> KPVIKMYQIGDKPDNLDELLANANKIIEEKVGAKLDIQYLGWGDYGKKMSVITSSGENYDIAFADNYIVNAQKGAYADLTELYKKEGKDLYKALDPAYIKGNTVNGKIYAVPVAANVASSQNFAF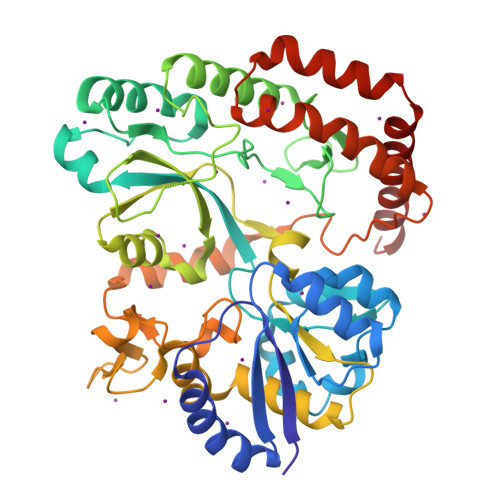NGTLLAKYGIDISGVTSYETLEPVLKQIKEKAPDVVPFAIGKVFIPSDNFDYPVANGLPFVIDLEGDTTKVVNRYEVPRFKEHLKTLHKFYEAGYIPKDVATSDTSFDLQQDTWFVREETVGPADYGNSLLSRVANKDIQIKPITNFIKKNQTTQVANFVISNNSKNKEKSMEILNLLNTNPELLNGLVYGPEGKNWEKIEGKENRVRVLDGYKGNTHMGGWNTGNNWILYINENVTDQQIENSKKELAEAKESPALGFIFNTDNVKSEISAIANTMQQFDTAINTGTVDPDKAIPELMEKLKSEGAYEKVLNEMQKQYDEFLKNKK[(2R,3R,4R,5R)-5-[[[[(2R,3S,4R,5R)-5-(6-aminopurin-9-yl)-3,4-bis(oxidanyl)oxolan-2-yl]methoxy-oxidanyl-phosphoryl]oxy-oxidanyl-phosphoryl]oxymethyl]-2,4-bis(oxidanyl)oxolan-3-yl] benzoate | C22 H27 N5 O15 P2 | 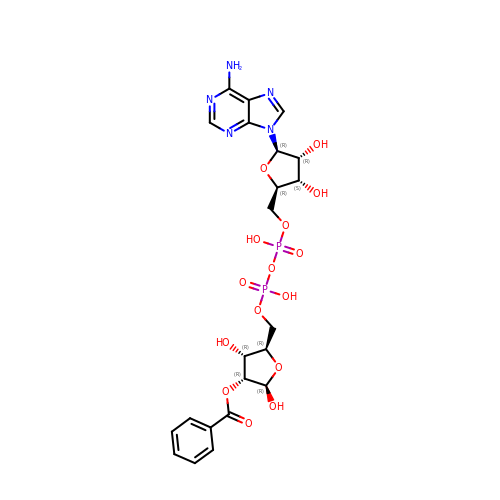MMZWJWZBUSRQKT-CJXJKIKOSA-N>[2x]MDEPDLKDLFITVDEPESHVTTIETFITYRIITKTSRGEFDSSEFEVRRRYQDFLWLKGKLEEAHPTLIIPPLPEKFIVKGMVERFNDDFIETRRKALH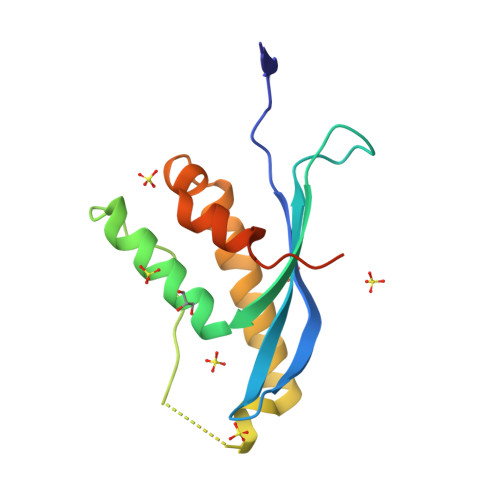KFLNRIADHPTLTFNEDFKIFLTAQAWELSSHAHHHHHH methyl (1R,3R)-1-methyl-3-[[3-[[3-methyl-4-[(4-pyridin-3-ylpyrimidin-2-yl)amino]phenyl]carbamoyl]phenyl]methylcarbamoyl]-4-oxidanylidene-cyclohexane-1-carboxylate 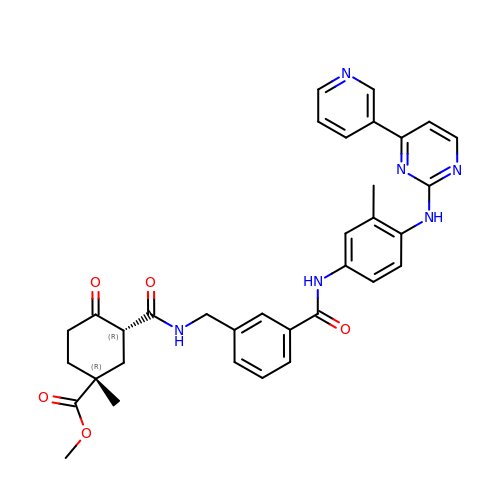| C34 H34 N6 O5 | GREBBMSDFQCEIO-OOXUFLSTSA-N>LGKFSQTCYNSAIQGSVLTSTCERTNGGYNTSSIDLNSVIENVDGSLKWQPSNFIETCRNTQLAGSSELA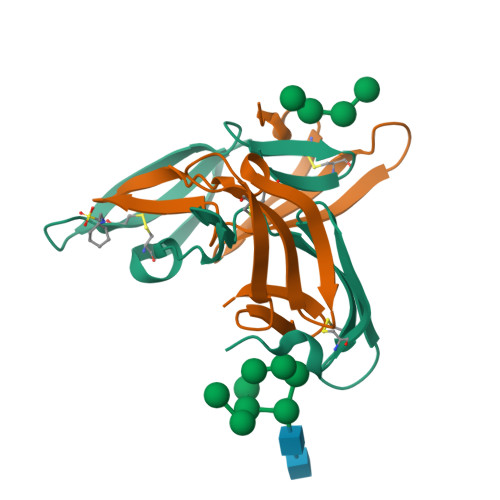AECKTRAQQFVSTKINLDDHIANIDGTLKYE[2x]>[2x]SRYIMGRTVLNESNKGLVENFSIPAELHERDGKRFASFGTTVPIHCCTPEQVAEFANKTHHYCDVFTEQVLAPLDELVYVRIDENTAEKVFINRSKRILLVSSDGVLAQWRSAPTFESSNRFLAGTPIVNKDGDLVSVVTARKGNHYAVSTFEGEGGYFETSQPWKVLDPPEGAAVYGDRWFPSREEVRAYTLSLPGAAVSAGSPPAPVLHRGGSGRLVLADARGRQLSHHYLHGVATTDVQYL

Poxviruses are large DNA viruses which replicate exclusively in the cytosol, and encode poxvirus immune nucleases (poxins) to degrade 2′3′-cGAMP and prevent STING activation (Eaglesham et al., 2019). While baculovirus and lepidopteran poxin homologs share <25% identity with VACV poxin, they are functional nucleases and retain 2′3′-cGAMP-specific cleavage activity. New poxin structures include the alphabaculovirus Autographa californica nucleopolyhedrovirus (AcNPV) poxin from Group 2, lepidopteran host poxins from the moth Trichoplusia ni and the monarch butterfly Danaus plexippus in Group 3, and the betabaculovirus Pieris rapae granulovirus (PrGV) poxin from Group 4. In spite of dramatic sequence divergence, poxin structures from each group reveal a shared core fold and head-to-tail dimeric architecture confirming poxins as a single enzyme family.

The new poxin structures trap a post-reaction state following 2′3′-cGAMP cleavage and allow direct comparison with the catalytic mechanism of VACV poxin. Unlike the catalytic triad of histidine, tyrosine, and lysine residues essential for VACV and AcNPV poxin cleavage activity, the active sites of T. ni poxin and PrGV poxin are divergent. The T. ni and PrGV poxin enzymes share the conserved active-site histidine but lack a tyrosine residue entirely. Instead, both proteins contain a second histidine residue adjacent to the first, which forms a contact with the 2′ hydroxyl or 3′ phosphate of the cleaved 2′3′-cGAMP molecule. In the case of T. ni poxin, mutagenesis analysis demonstrates this second histidine residue is essential for activity, suggesting this residue functions as a general base to deprotonate and activate the 2′ hydroxyl nucleophile for in-line cleavage of the 3′–5′ bond. Further, the T. ni poxin protein shows substitution of the VACV lysine for an arginine residue, whereas the lysine is conserved in PrGV poxin. Unlike mutation of the lysine residue in the VACV and AcNPV active sites, mutation of the T. ni poxin active-site arginine to alanine only partially reduces activity, and a charge-preserving mutation of the arginine to lysine results in even less activity. Analysis of the host T. ni poxin structure confirms a relationship with protease enzymes and demonstrates strong homology with proteases derived from (+)ssRNA viruses. Unlike the degenerated domain in VACV poxin, comparison of the N-terminal domain of T. ni poxin with the yellow fever virus protease demonstrates near complete conservation of a dual Greek key β-barrel fold common to serine protease enzymes. A nearly identical pocket is conserved on the surface of the T. ni poxin protease-like domain, in which the poxin C-terminus is also coordinated by histidine and aspartic acid residues.Ceftaroline, 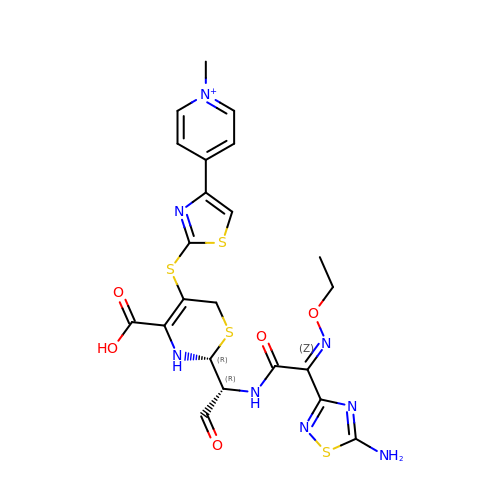bound form | C22 H23 N8 O5 S4 | QFDBBFVVRSTDES-CWTRNNRKSA-N> GEFLATTLERIEKNFVITDPRLPDNPIIFASDSFLQLTEYSREEILGRNCRFLQGPETDRATVRKIRDAIDNQTEVTVQLINYTKSGKKFWNLFHLQPMRDQKGDVQYFIGVQLDGTEHVRDAAEREGVMLIKKTAENIDEAAKEL

Light-oxygen-voltage (LOV) proteins form a sensory photoreceptor class that elicit a wide palette of physiological responses to blue light across archaea, bacteria, protists, fungi, and plants. Likely via a radical-pair mechanism, T1 reacts within microseconds to the signaling state, characterized by a covalent thioadduct between a highly conserved cysteine residue in the LOV photosensor and the C4a atom of the flavin isoalloxazine ring system. Thioadduct formation entails a hybridization change of the flavin C4a atom from sp2 to sp3 and concomitant protonation of the adjacent N5 atom. A highly conserved glutamine residue in strand Iβ is situated immediately adjacent to the flavin and has been identified as instrumental in reading out the flavin N5 position and eliciting the downstream transitions.

To arrive at a molecular understanding, we solved the crystal structures of AsLOV2 wild-type and Q513L in the dark-adapted states to resolutions of 1.00 Å and 0.90 Å, respectively. The flavin pteridin moiety was coordinated by the asparagines N482 and N492, and the flavin O4 atom hydrogen-bonded to the amide NεH2 group of the conserved Q513. At the present high resolution, an alternate conformation could be resolved for the terminal turn of the Jα helix (residues 543-546), possibly reflecting the inherent equilibrium between folded and unfolded helical states. Crucially, the A’α helix is interlocked with the C-terminal part of Jα via the hydrophobic residues L408, I411, I539, A542, and L546.> GAMAEQQLRLPSPEVYRFVVKDSEENIVFEDNLQSRSGIPIIKGGTVVKLIERLTYHMYADPNFVRTFLTTYRSFCKPQELLSLLIERFEIPEPEPTDADKLAIEKGEQPISADLKRFRKEYVQPVQLRILNVFRHWVEHHFYDFERDLYLLERLESFISSVRGKAMKKWVESIAKIIRRKKQAQANGVSHNITFASPPPPIEWHISKPGHIETFDLMTLHPIEIARQLTLLESDLYRKVQPSELVGSVWT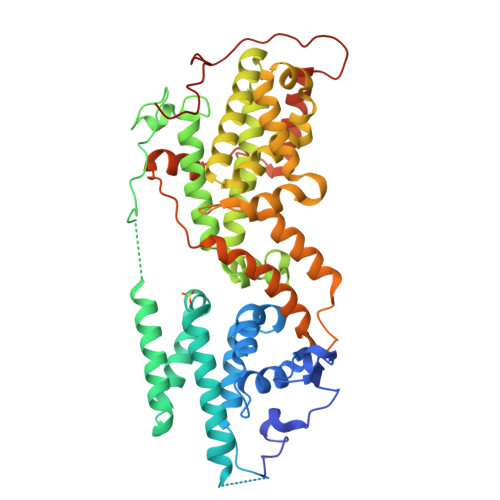KEDKEINSPNLLKMIRHTTNLTLWFEKCIVEAENFEERVAVLSRIIEILQVFQDLNNFNGVLEIVSAVNSVSVYRLDHTFEALQERKRKILDEAVELSQDHFKKYLVKLKSINPPCVPFFGIYLTNILKTEEGNNDFLTRHGKDLINFSKRRKVAEITGEIQQYQNQPYCLRIEPDMRRFFENLNPMGSASEKEFTDYLFNKSLEIEPRNPKQPPRFPRKSTFSLKSPGIRPNTGRHGS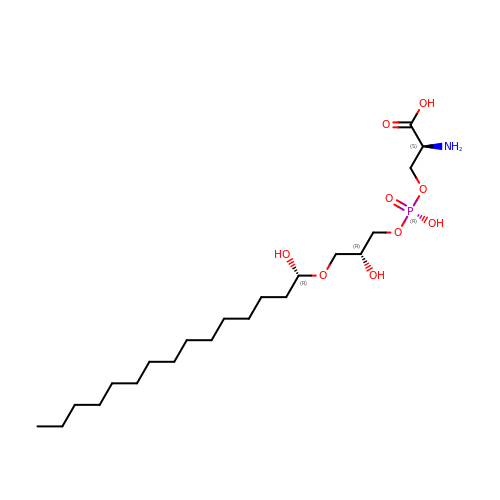O-{HYDROXY[((2R)-2-HYDROXY-3-{[(1S)-1-HYDROXYPENTADECYL]OXY}PROPYL)OXY]PHOSPHORYL}-L-SERINE | C21 H44 N O9 P | RPZLJDFLPRHXGM-HSALFYBXSA-N>MFTGSIVAIVTPMDEKGNVCRASLKKLIDYHVASGTSAIVSVGTTGEWATLNHDEHADVVMMTLDLADGRIPVIAGTGANATAEAISLTQRFNDSGIVGCLTVTPYYNRPSQEGLYQHFKAIAEHTDLPQILYNVPSRTGCDLLPETVGRLAKVKNIIGIKEATGNLTRVNQIKELVSDDFVLLSGDDASALDFMQLGGHGVISVTANVAARDMAQMCKLAAEGHFAEARVINQRLMPLHNKLFVEPNPIPVKWACKELGLVATDTLRLPMTPITDSGRETVRAALKHAGLL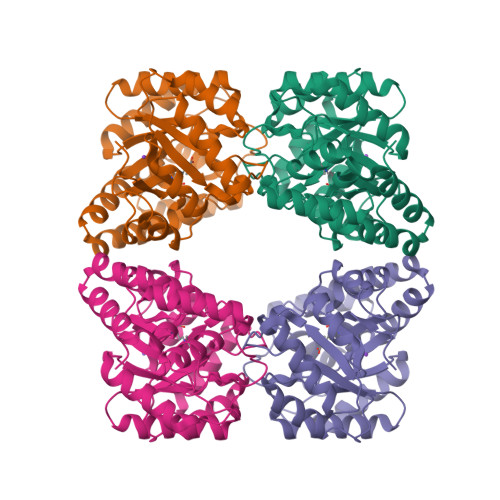[2x]>[2x]MATVEPETTPTPNPPTTEEEKTESNQEVAN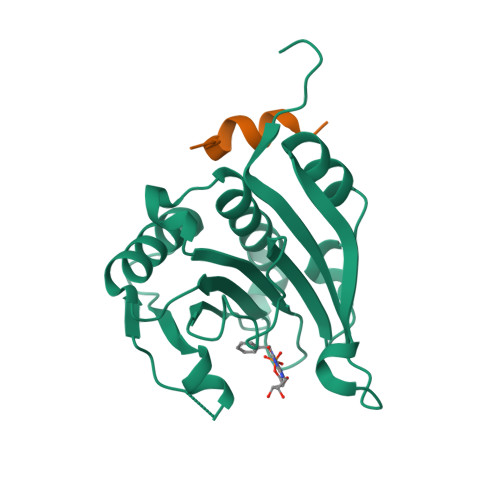PEHYIKHPLQNRWALWFFKNDKSKTWQANLRLISKFDTVEDFWALYNHIQLSSNLMPGCDYSLFKDGIEPMWEDEKNKRGGRWLITLNKQQRRSDLDRFWLETLLCLIGESFDDYSDDVCGAVVNVRAKGDKIAIWTTECENREAVTHIGRVYKERLGLPPKIVIGYQSHADTATKSGSTTKNRFVV;>[2x]RIIYDRKFLMECRN> GSTGGVQTVTLIPGDGIGPEISAAVMKIFDAAKAPIQWEERNVTAIQGPGGKWMIPSEAKESMDKNKMGLKGPLKTPIAAGHPSMNLLLRKTFDLYANVRPCVSIEGYKTPYTDVNIVTIRENTEGEYSGIEHVIVDGVVQSIKLITEGASKRIAEFAFEYARNNHRSNVT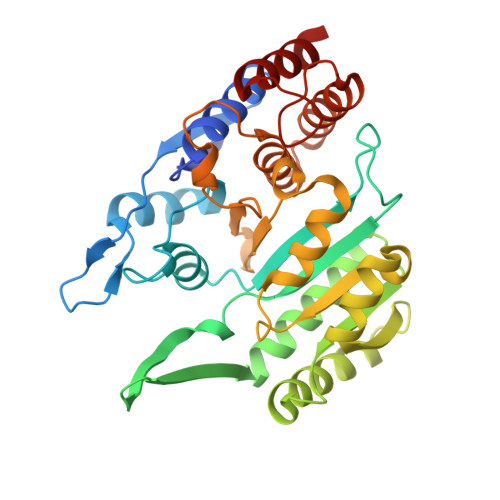AVHKANIMRMSDGLFLQKCREVAESCKDIKFNEMYLDTVCLNMVQDPSQFDVLVMPNLYGDILSDLCAGLIGGLGVTPSGNIGANGVAIFESVHGTAPDIAGKDMANPTALLLSAVMMLRHMGLFDHAARIEAACFATIKDGKSLTKDLGGNAKCSDFTEEICRRVKDLD>[2x]GSHMSTPARRRLMRDFKRMKEDSPPGVSASPLPDNVMIWNAMIIGPADTPYEDGTFRLLLEFDEEYPNKPPHVKFLSEMFHPNVYANGEICLDILQNRWTPTYDVASILTSIQSLFNDPNPASPANVEAATLFQDHKSQYVKRVKETVEKSWEDDMEDMADEDEDEE;>[4x]MNDHFVKRPKLELSDPSEPLTQKDVIAFQKEALFRCLNKWRVKANQLVEENEVLAA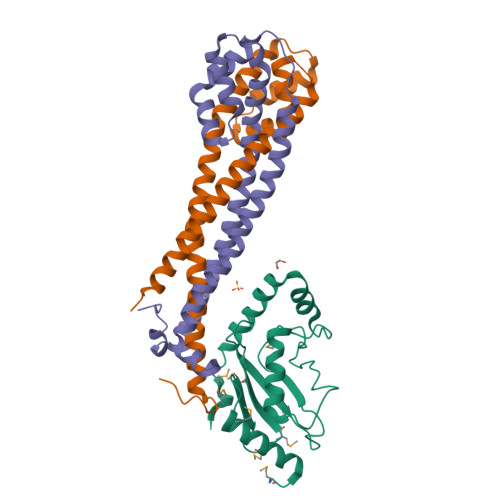GLSKTTESVSGCCSSIVVLARSVVEDCSDEQDKRFLQQLINTEDEHTLTQIISNNSARICELILKTSGSNISDNIGRLQELESLTLTLQKLLKSSENKLKKATEYYENIIAQYDRQDSESVSRVFNTADDDSNVKKEKQSSTGASSVNDE>[4x]MKVLGVVVEYNPFHNGHLYHLTSARELVKPDYTIAVMSGNFCQRGEPAVIDKFARAEIALRMGVDVVLELPVVFATQDAGGFAFGAVCVLDATGVVTDVVFGS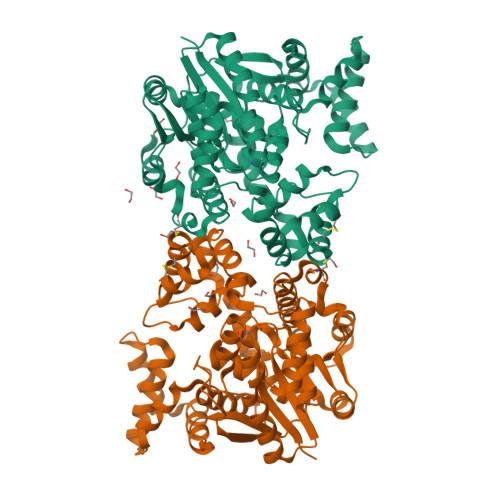ESNDIEFLQRVARILYEQPDEYQKFLHEELKKGYSFPNARKYALMRYFSMKGWNEEEVLKLEKSNDILGVEYIHSALKIGSNIRFHTIKRVGAEEKDTSFRGRFSSATAIRNLMREKRWEEVRDSLPEDSFEILMREINEGRGPVFLENMGDFLLSFFRLKNMDFFEKIHGFSEGLEKRFHVCARQTGSYRDFLECVKAKRFTFSRIRRLALFSVFEVNKEFVEKSNTKGPQYIRILGFTEKGREILSLMRKKAKLPIVTNMSLYRKVLEKTDLPVDKQLFLEQIDLDVKATNFYSMFFPSVEQRCGERDFSIHPIFLRTEM>[4x]QAGFDLLNDGRPETLWLGIGTLLMLIGTFYFIARGWGVTDKEAREYYAITILVPGIASAAYLAMFFGIGVTEVELASGTVLDIYYARYADWLFTTPLLLLDLALLAKVDRVTIGTLIGV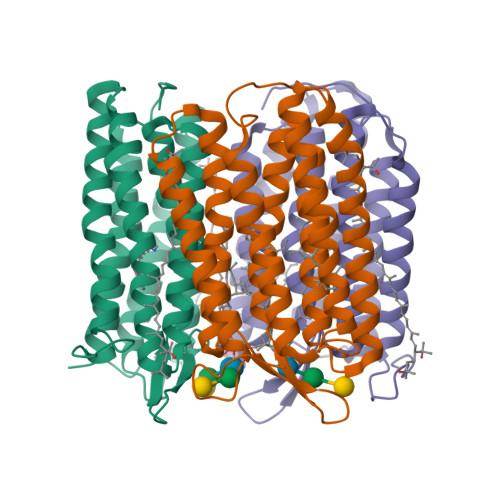DALMIVTGLIGALSKTPLARYTWWLFSTIAFLFVLYYLLTSLRSAAAKRSEEVRSTFNTLTALVAVLWTAYPILWIVGTEGAGVVGLGIETLAFMVLDVTAKVGFGFVLLRSRAILGETEAPEPSAGADASAAD> DPSKDSKAQVSAAEAGITGTWYNQLGSTFIVTAGA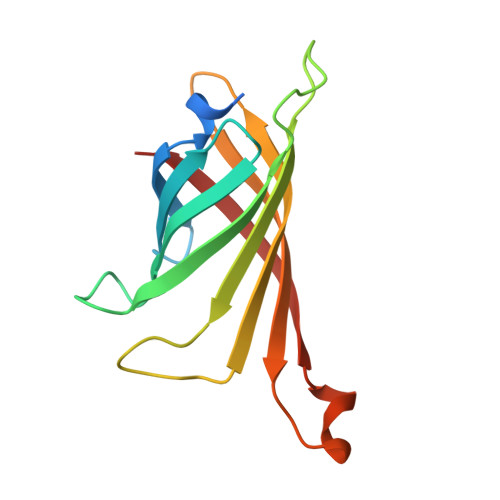DGALTGTYESAVGNAESRYVLTGRYDSAPATDGSGTALGWTVAWKNNYRNAHSATTWSGQYVGGAEARINTQWLLTSGTTEANAWKSTLVGHDTFTKVKP The process is initiated by the mitochondrial core ISC complex, which synthesizes a [2Fe-2S] cluster de novo from cysteine-derived sulfur and ferrous iron (Fe2+). This complex is composed of the iron-sulfur scaffold protein ISCU2, the dimeric pyridoxal phosphate (PLP)-dependent cysteine desulfurase subcomplex NFS1-ISD11-ACP1, the allosteric regulator frataxin (FXN), and the electron donor ferredoxin-2 (FDX2), which is itself reduced by the NADPH-dependent ferredoxin reductase (FDXR). The sulfane sulfur (S0) of the persulfide on ISCU2 is reduced to sulfide (S2-) by FDX2 to initiate [2Fe-2S] cluster formation. FDX2 and FXN compete for binding to overlapping sites at the core ISC complex during de novo [2Fe-2S] cluster biosynthesis.

First, to elucidate the interaction site of reduced FDX2 with the (NIAU)2 complex, the (NIA)2 subcomplex was incubated for 20 min with iron-loaded ISCU2 and FDXR-reduced FDX2 to yield the (NIAUF)2 sample. In the (NIAUF)2 dataset, 61% of the particles belong to a class in which FDX2 is bound in the proximal conformation, and 39% belong to a distal-bound FDX2 class. Additional weak density at this site, typically associated with conformational and/or compositional heterogeneity in cryo-EM, was further assessed by C2 symmetry expansion and focused 3D classification. This revealed two major FDX2 conformations that we refer to as ‘proximal’ and ‘distal’ according to the distances between the [2Fe-2S] cluster of FDX2 and the FeS cluster assembly site of ISCU2, namely 23 Å for the distal conformation and 14 Å for the proximal conformation. In the distal conformation, the [2Fe-2S] cluster of FDX2 is too far for efficient electron transfer to the ISCU2 FeS cluster assembly site (23 Å), whereas the movement to the proximal binding position brings the [2Fe-2S] cluster to a distance of 14 Å that would allow rapid electron transfer for reduction of the Cys138ISCU2 persulfide. When bound in the proximal position, the C terminus of FDX2 is ordered and well resolved, interacting extensively with the NFS1 subunit. Contact is mediated by hydrogen bonds (H-bonds) between Asn175FDX2 and Cys-loop Ser385NFS1, a salt bridge between Asp179FDX2 and Arg393NFS1 and hydrophobic interactions of Phe176FDX2 and Val178FDX2 with Leu160NFS1. When FDX2 is bound in the proximal position, the H-bonds between Asn175FDX2 and Ser385NFS1 could provide additional stability for the ‘outward’ Cys-loop conformation. Residue His186FDX2 is resolved only in the proximal conformation of our (Fe-NIAUF)2 structure, yet does not interact with other residues in this complex. The movement is achieved by a rearrangement and tightening of the salt bridges between NFS1’ and FDX2.

>[2x]MSLRPLYMDVQATTPLDPRVLDAMLPYLINYYGNPHSRTHAYGWESEAAMERARQQVASLIGADPREIIFTSGATESNNIAIKGVARFYRSRKKHLITTQTEHKCVLDSCRSLEAEGFQVTYLPVQKSGIIDLKELEAAIQPDTSLVSVMTVNNEIGVKQPIAEIGRICSSRKVYFHTDAAQAVGKIPLDVNDMKIDLMSISGHKIYGPKGVGAIYIRRRPRVRVEALQSGGGQERGMRSGTVPTPLVVGLGAACEVAQQEMEYDHKRISKLSERLIQNIMKSLPDVVMNGDPKHHYPGCINLSFAYVEGESLLMALKDVALSSGSACTSASLEPSYVLRAIGTDEDLAHSSIRFGIGRFTTEEEVDYTVEKCIQHVKRLREMSPLWEMVQDGIDLKSIKWTQH;>MGSSHHHHHHGSPTTENLYFQGHNMAASSRAQVLALYRAMLRESKRFSAYNYRTYAVRRIRDAFRENKNVKDPVEIQTLVNKAKRDLGVIRRQVHIGQLYSTDKLIIENRDMPRT[2x];>MSTIEERVKKIIGEQLGVKQEEVTNNASFVEDLGADSLDTVELVMALEEEFDTEIPDEEAEKITTVQAAIDYINGHQA[2x];>MAYHKKVVDHYENPRNVGSLDKTSKNVGTGLVGAPACGDVMKLQIQVDEKGKIVDARFKTFGCGSAIASSSLATEWVKGKTVEEALTIKNTDIAKELCLPPVKLHCSMLAEDAIKAALADYKLKQEPKKGEAEKKLEHHHHHH[2x];> MASDVVNVVFVDRSGQRIPVSGRVGDNVLHLAQRHGVDLEGACEASLACSTCHVYVSEDHLDLLPPPEEREDDMLDMAPLLQENSRLGCQIVLTPELEGAEFTLPKITRNFYVDGHVPKPH> GKITLYEDRGFQGRHYECSSDHPNLQPYLSRCNSARVDSGCWMLYEQPNYS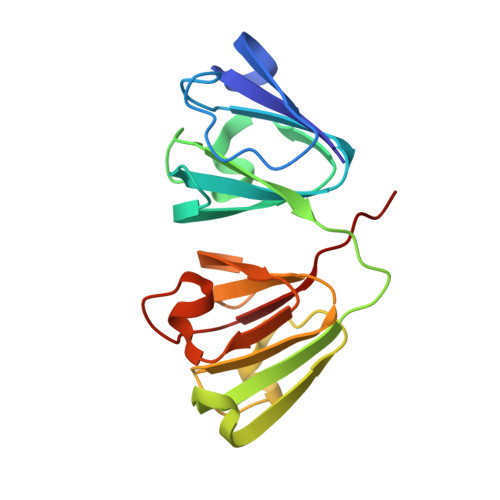GLQYFLHRGDYADHQQWMGLSDSVRSCRLIPHSGSHRIRLYEREDYRGQMIEFTEDCSCLQDRFRFNEIHSLNVLEGSWVLYELSNYRGRQYLLMPGDYRRYQDWGATNARVGSLRRVIDFS1-CYCLOHEXYL-3-METHYL-UREA | C8 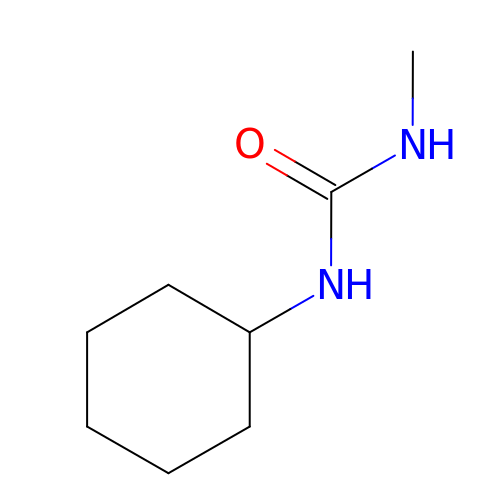H16 N2 O | YKLDLMXTBHWMPV-UHFFFAOYSA-N Cellvibrio japonicus is a saprotrophic bacterium which possesses the remarkable ability to grow in isolation using a variety of hemicellulosic polysaccharides as sole carbon sources. It produces a diverse collection of GHs, assembling enzyme systems that can degrade cellulose, xylans, mannans, and xyloglucans, among others. Effective xyloglucan-degrading GH systems (recently reviewed by Attia and Brumer) contain exo-acting glycosidases acting as debranching accessory enzymes and endo-acting enzymes (xyloglucanases) that generate short, branched β-(1,4)-glucan oligomers (xyloglucan oligosaccharides).18−23Exo-acting enzymes are expected to address each of the glycosidic linkages reported in xyloglucan branches, though the reported enzyme diversity falls short of reported branch diversity. The work presented here comprises the design and validation of trisaccharidic xyloglucan (“XyG”)-type cyclophellitol probes and their validation as bona fide, predictive tools for the identification of xyloglucanase activities and their discrimination from cellulase activities within a xyloglucan-elicited C. japonicus degradome.

Not having been previously functionally or structurally characterized in detail, we produced and purified Cel5B and Cel5C recombinantly in E. coli to assess further the correlation between probe reactivity and enzyme specificity. We found that Cel5B and Cel5C were both cellulases, efficiently degrading carboxymethylcellulose and mixed-linkage β-glucan. Cel5B showed only weak activity toward tamarind xyloglucan while Cel5C had weak activity toward carob galactomannan and no detectable xyloglucanase activity. To determine the molecular basis for the reactivity of ABP-XyG-Cy5 with CjCel5B but not CjCel5C, we crystallized both enzymes and solved their structures by molecular replacement in both unliganded and ABP-bound forms. Notably, the active site cleft of CjCel5B is significantly more open beyond the −2 subsite, so we hypothesized that cellulase-specificity in Cel5B is dictated primarily by an inability to accommodate α-(1,6)-xylose residues in the positive subsites. We also observed that growth on glucose resulted in low-level expression of Cel5B, while growth on xyloglucan resulted in expression of Cel5D correlating with a decrease in observed Cel5B activity, suggesting that Cel5B is acting as a “sensing” enzyme that is repressed by the detection of xyloglucan. Extending this analysis to xyloglucan-grown cell lysate yielded a complex pattern of apparent glycoproteins, including a band at the position of Cel5D. Intact mass of the purified Cel5B measured via denaturing LC-ESI-MS gave a protein peak with a series of deconvoluted mass values from 71 to 75 kDa with spacing of 162 Da, indicating heavy glycosylation with variable hexose content (Supplemantal Figure 29). Considering the intact MS and monosaccharide composition, we propose that the underlying glycan structure is a galactoglucomannan O-glycan.

> MVAPLSVQGNKILANGQPASFSGMSLFWSNTEWGGEKYYNAQVVSWLKSDWNAKLVRAAMGVEDEGGYLTDPANKDRVTQVVDAAIANDMYVIIDWHSHNAHQYQSQAIAFFQEMARKYGANNHVIYEIYNEPLQVSWSNTIKPYAQAVIAAIRAIDPDNLIIVGTPTWSQDVDVAANDPITGYQNIAYTLHFYAGTHGQYLRDKAQTALNRGIALFVTEWGSVNANGDGAVANSETNAWVSFMKTNHISNANWALNDKVEGASALVPGASANGGWVNSQLTASGALAKSIISGWPSYLEHHHHHH> GSEAAGGEQRELLIQR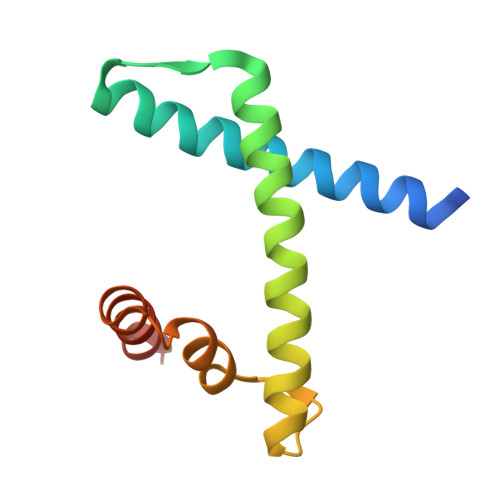LRAAVHYTTGALAQDVAEDKGVLFSKQTVAAISEITFRQAENFARDLEMFARHAKRSTITSEDVKLLARRSNSLLKYITQKSDELASSNME> SIVTKSIVNADAEARYLSPGELDRIKSFVSGGAQRLRI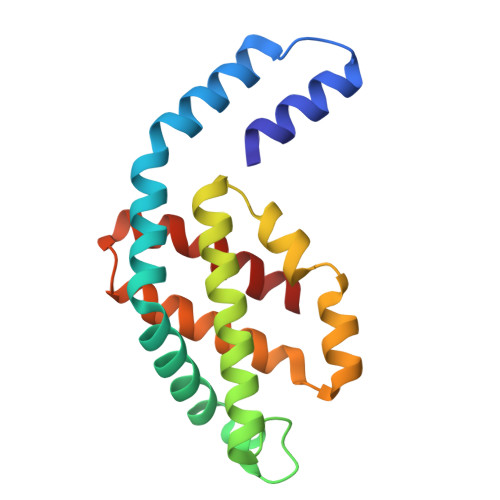AQVLTDNRERIVKQAGDQLFQKRPDVVSPGGNAYGQEMTATCLRDLDYYLRLVTYGIVAGDVTPIEEIGIVGVREMYKSLGTPIDAVAGGVAAMKSVAAGLLSAEDAGEAGAYFDYVVGAMQ>NAMARKKITLVGAGNIGGTLAHLALIKQLGDVVLFDIAQGMPNGKALDLLQTCPIEGVDFKVRGTNDYKDLENSDVVIVTAGVPRKPGMSRDDLLGINIKVMQTVGEGIKHNCPNAFVICITNPLDIMVNMLQKFSGVPDNKIVGMAGVLDSARFRTFLADELNVSVQQVQAYVMGGHGDTMVPLTKMSNVAGVSLEQLVKEGKLK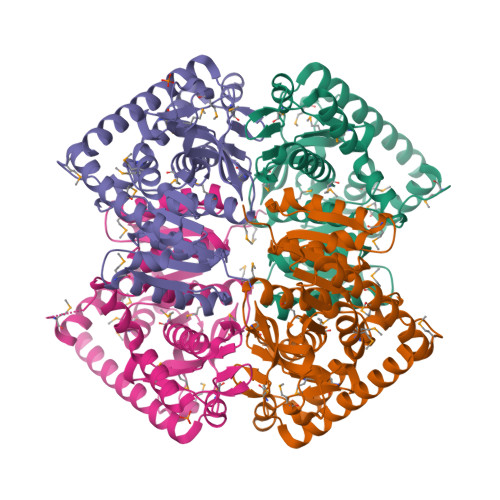QERLDAIVSRTRSGGGEIVALLKTGSAYYAPAAAGIQMAESFLKDKKMILPCAAKVKAGMYGLDEDLFVGVPTEISANGVRPIEVEISDKEREQLQVSINAIKDLNKAAAEILAK[4x]> MAHHHHHHMIRE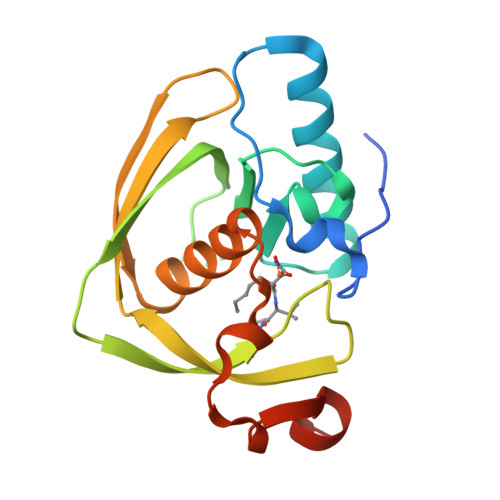ILKMGDPRLLEVARPVDRFDTPELHEIVADMFETMHHANGAGLAAPQIGIGLQIIIFGFGSNDRYPDAPPVPETVLINPKLEYMPPDMEEGWEGCLSVPGMRGVVSRYAKVRYSGFDQFGAKIDRVAEGFHARVVQHEYDHLIGKLYPMRITDFTRFGFTEVLFPGLDPAADD> AFLILVIGNLHIPDRALDIPPKFKKLLS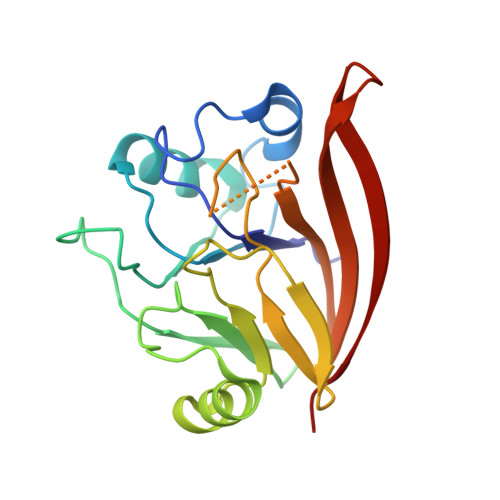PGKISQTLCLGNLTDRATYDYLRSISPDLKIVRGRMDVEATSLPLMQVVTHGSLRIGFLEGFTLVSEEPDVLLAEANKLDVDVLCWAGGSHRFECFEYMDKFFVNPGSATGAFTTDWLAEGEEVVPSFCLMDVQGISLTLYVYQLRKDENGTENVAVEKVTYTKP> NYIVPGEYRVAEGEIEINAGREKTTIRVSNTGDRPIQVGSHIHFVEVNKELLFDRAEGIGRRLNIPSGTAARFEPGEEMEVELTELGGNREVFGIS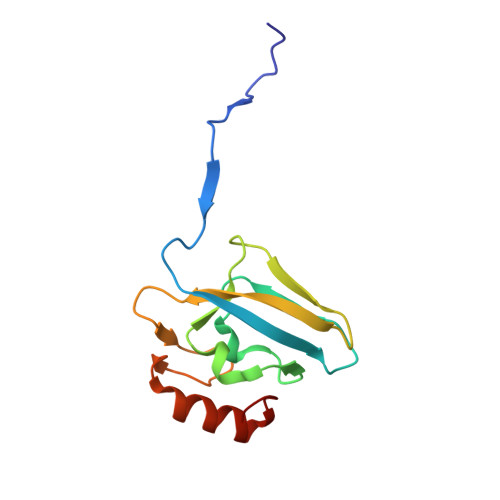DLTNGSVDNKELILQRAKELGYKGVE However, exceptionally high-level aminoglycoside-resistance is achieved by the action of intrinsic and acquired 16S ribosomal RNA (rRNA) methyltransferase enzymes in aminoglycoside-producing and human pathogenic bacteria, respectively. These resistance determinants block drug binding by catalyzing the transfer of a methyl group from their cosubstrate S-adenosyl-l-methionine (SAM) to the base of a defined target RNA nucleotide within the ribosomal A-site. Here, we describe detailed structural and functional analyses of one of these enzymes, the kanamycin-resistance methyltransferase from Catenulisporales acidiphilia (‘CacKam’). CacKam has a SAM-binding core fold comprised of a seven-stranded β-sheet with a central topological switch point, characteristic of Class I methyltransferases.

However, a 2.7 Å resolution structure of the CacKam-SAH complex was obtained by soaking preformed crystals of apo CacKam with SAH. This complex structure revealed that the SAM-binding pocket is largely preformed in the apo protein. While the β6/7 linker does not undergo a complete reorganization to a structure resembling that of KamB or NpmA which caps the SAM-binding pocket, SAH binding nonetheless appears to induce greater β6/7 linker flexibility reflected by significantly higher B-factors relative to the remainder of the protein, which is essentially unchanged. Binding of SAH to wild-type CacKam is accommodated by a small (∼1.5 Å) repositioning of the protein backbone encompassing the conserved GxGx(G) motif (38GTGDA42 in CacKam). The G38 backbone carbonyl forms a hydrogen bond with the SAH amino group, which is additionally positioned by two conserved residues, via hydrogen bonding interaction with the L110 backbone carbonyl group and a water-mediated interaction with the side chain of D36. As the β6/7 linker remains in an extended conformation in the CacKam-SAH structure, interaction with the SAH carboxyl group is limited to a single hydrogen bonding interaction with S201. The hydroxyl groups of the SAH ribose moiety form two hydrogen bonds with the highly conserved aspartic acid residue, D61, while the adenine base is bound in a hydrophobic pocket formed by residues L116, I93 and P62, and additionally positioned by a hydrogen bond between the adenine N6 and the side chain of CacKam residue E94. Conserved hydrophobic and hydrogen bonding interactions are made with the adenine base, ribose and homocysteine moiety of SAH.

> MHHHHHHASGLVPRGSHMTRTTALKVLAGKKLTDLDPDEWAKAQASAERILVDVGTGDARTAYRQAIAHPEWLVVGVDPAWQRMTETAVRAARKPAKGGAPNLVLVSSAIETVPAALHGVADEVMVLMPWGKLLRGVVLGEADVLSGLRAVAKPGAPLEISIGTSIWREPIPLEIRDLPELTPETVVSTGLTDRLAALGWQVADVRLVPHTDLDTISSSWARRLGSGATETVLHLRAVAVDPRDPVGTQHPAAESAQDTPEEPQRDV Salinixanthin 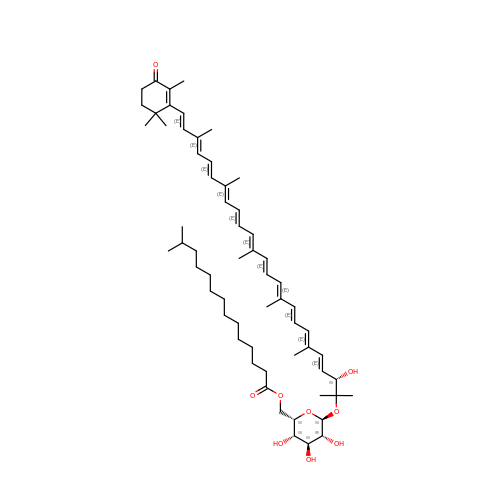| C61 H92 O9 | BUNXUZXQWPTVHM-CRAPJSHNSA-N> QPSRKEKSLGLLCHKFLARYPNYPNPAVNNDICLDEVAEELNVERRRIYDIVNVLESLHMVSRLAKNRYTWHGRHN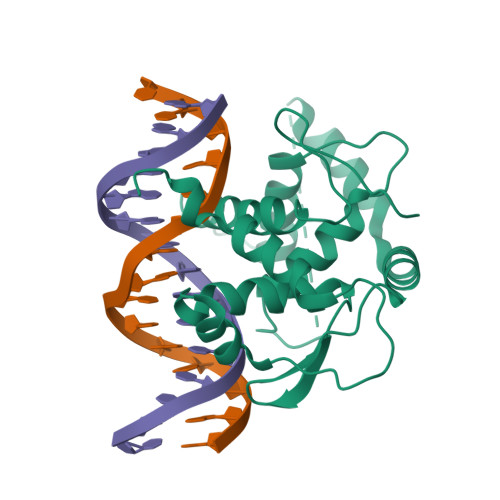LNKTLGTLKSIGEENKYAEQIMMIKKKEYEQEFDFIKSYSIEDHIIKSNTGPNGHPDMCFVELPGVEFRAASVNSRKDKSLRVMSQKFVMLFLVSTPQIVSLEVAAKILIGEDHVEDLDKSKFKTKIRRLYDIANVLSSLDLIKKVHVTEERGRKP> GSDEYDYLFKVVLIGDSGVGKSNLLSRFTRNEFNLESKSTIGVEFATRSIQVDGKTIKAQIWDTAGLER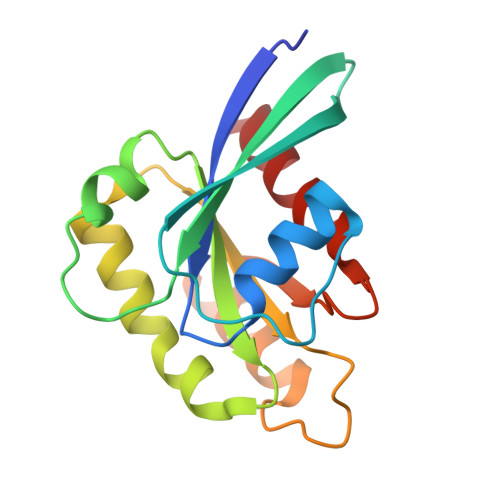YRAITSAYYRGAVGALLVYDIAKHLTYENVERWLKELRDHADSNIVIMLVGNKSDLRHLRAVPTDEARAFAEKNGLSFIETSALDSTNVEAAFQTILTEIYRI>[4x]MHHHHHHENLYFQGASVLVASNRGPVSYVRGEDGELDARRGGGGLVSGLSAVSSQDSLWVCAALGEGDREAVRRGIGEPGVRMLDIAPDVYADAYNGIANSVLWFLHHHLYDIPREPVFDAAFRHRWEAYRAYNRAFAEALAAAADEGAAVLVQ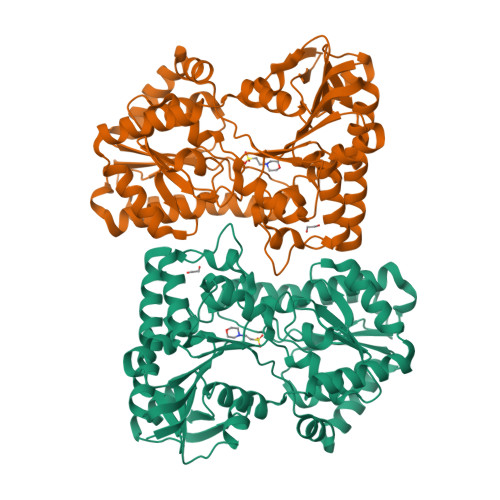DYHLALVPGQLRELRPDLRIGHFTHTPWASPEYFRMLPADIGDELLRGMLGADELGFHTSAWASAFLSCAGGEQPRTRVRVHPLGVDAEELRALAHRPQVDERLARLREEVGDRKTIVRVDRTELSKNILRGLLAYRELLTVHPEWRDRVVHLASAYPSRQDLAAYRAYTASVTELAAEINAEFGTADWQPVLVSVEDDFTRSLAAYRLADVALVNPVRDGMNLVAKEIPVVSDAGCALVLSTGAGAYEELKEDALTVHPYDVSETAEALHTALTMPPPERADRTKRLASAATALPPQRWFLNQLEGLSDA> MSWALEMADTFLDNMRVGPRTYADVRDEINKRGREDREAARTAVHDPERPLLRSPGLLPEIAPNASLGVVHRRT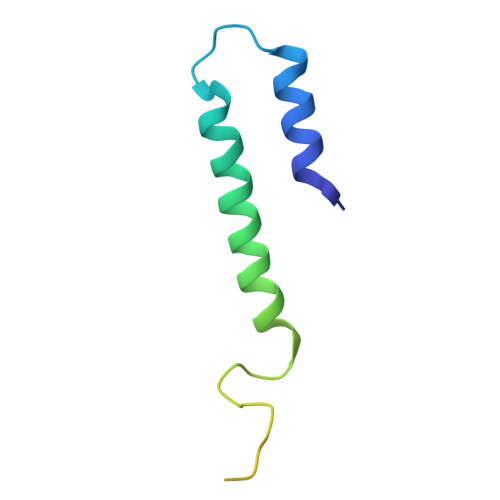GGTVTDSPRNPVTR> MAHTAAERPPEETLSLWKGEQARLKARVVDRDTEAWQRDPSFSGLQKVGGVAVSFVKGDSVRACASLVVLSYPELKVVYEDSRMVGLKAPYVSGFLAFREVPFLVELVQRLQEKEPDLMPQVVLVDGNGVLHQRGFGVACHLGVLTELPCIGVAKKLLQVDGLENNALHKEKIVLLQAGGDTFPLIGSSGTVLGMALRSHDHSTKPLYVSVG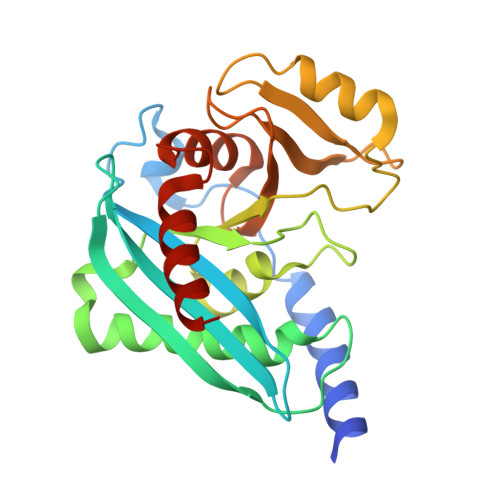HRISLEVAVRLTHHCCRFRIPEPIRQADIRSREYIRRT Initially, the 40S ribosomal subunit associates with Met-tRNAi and a group of initiation factors, including eIF1, eIF1A, eIF2, eIF3, and eIF5 to form the 43S pre-initiation complex. This complex is then recruited to the 5′-end of capped mRNA by another complex of factors (known as eIF4F) consisting of eIF4E, eIF4G, and eIF4A. eIF4E is an indispensable element for cap-dependent translation initiation and plays a major role in recognition of the mRNA cap structure (m7GpppN, where N is any nucleotide). Under resting conditions, eIF4E is kept in an inactive form bound to 4E-binding proteins (4E-BPs); once the latter have been phosphorylated through the PI3K-AKT-mTOR signalling pathway, eIF4E is released and can associate with eIF4G to launch translation. eIF4E is overexpressed in numerous human tumours, and it contributes to transformation, tumourigenesis, and progression of cancers. eIF4E overexpression facilitates translation of weak and highly structured mRNAs that typically encode proteins involved in cancer pathology, such as proto-oncoproteins (e.g. cyclin D1, ornithine decarboxylase), angiogenesis factors (e.g. FGF-2, VEGF), and factors related to tumour invasiveness, such as MMP-9, due to the ability of eIF4E to stimulate eIF4A. All complex structures showed the characteristic cupped hand structure of eIF4E with the ligands occupying the cap-binding site.

Squaric acid possesses similar charge distribution, polarity, and acidic properties as phosphoric acid, hence the squaramide group could represent an isostere for the phosphate group. Despite low overall resolution, the eIF4E co-crystal structure with ligand 4a clearly shows that the squaramide moiety acts as a phosphate mimic by making a similar interaction with R157 despite an altered conformation. The positively charged N7-methyl guanine system forms the characteristic cation-π interaction as expected. Surprisingly, in the context of the squaramide phosphomimetic group, the expected enhancement of affinity upon replacing the N7-methyl group (4a) with a benzyl group (4b) was not observed. Crystal structures of sulfonamide 7a and squaramides 4a and 4f in complex with eIF4E were obtained and show similar binding modes to cap derivatives co-crystallised with eIF4E previously.

>MATVEPETTPTPNPPTTEEEKTESNQEVANPEHYIKHPLQNRWALWFFKNDKSKTWQANLRLISKFDTVEDFWALYNHIQLSSNLMPGCDYSLFKDGIEPMWEDEKNKRGGRWLITLNKQQRRSDLDRFWLETLLCLIGESFDDYSDDVCGAVVNVRAKGDKIAIWTTECENREAVTHIGRVYKERLGLPPKIVIGYQSHADTATKSGSTTKNRFVV[2x];>RIIYDRKFLMECRN[2x]>[4x]MPVPNGATFPPCARKMERADGPATVLAIGTANPPNVFDQSTYPDFYFNITNSNHMTDLKTKFQRMCDKSGITKRYMYLNEEILKANPNMCAYWEKSLDVRQDMVVVEVPKLGKEAATKAIKEWGQPKSKITHVVFCTTSGVDMPGADWALTKLLGLRPSVKRLMMYQQGCFAGGTVMRVAKDLAENNKGARVLVVCSELTAVTFRGPSETHLDSLVGQALFGDGASAIIVGADPIPEVERPWFEIHYVASNILPDSDGAIDGHLREVGLTFHLMKDVPGIISKNIGTVLKDAFEKVFGNEEGEVPSYNDVFWIAHPGGPAILDQVEQKLQLKTEKMAASRQVLSDYGNMSSACVLFIMDHLRKKSVEQKLATSGEGYEWGLLLGFGPGLTCETVVLRSVPLATE

Chalcone synthase, a well-studied ubiquitous plant-specific type III polyketide synthases (PKSs), is the first key enzyme in the flavonoid biosynthetic pathway. The biosynthesis of flavonoids starts with the condensation of one molecule of p-coumaryl CoA with three molecules of malonyl-CoA through the catalysis of chalcone synthase (CHS) to generate naringenin chalcone. Functional characterization of two chalcone synthases (CpCHS1 and CpCHS2) indicated that CpCHS1 can catalyze the formation of pinocembrin, naringenin, and eriodictyol, respectively; however, CpCHS2 was inactive. The crystallization investigation of CpCHS1 indicated that it has a highly similar conformation and shares a similar general catalytic mechanism to other plants CHSs.

The crystal structure of CpCHS1 was elucidated in the apo and presence of its final product naringenin, and detailed structural comparisons of CpCHS1 with EaCHS from Equisetum arvense and PpCHS from Physcomitrella patens revealed common differences between CHSs in the local conformation around the active site pocket. Mutation of several residues around the catalytic pocket of CpCHS1 dramatically reduced the in vitro catalytic activity of the enzyme, experimentally supporting their functional roles in substrate binding.METHOTREXATE | C20 H22 N8 O5 | 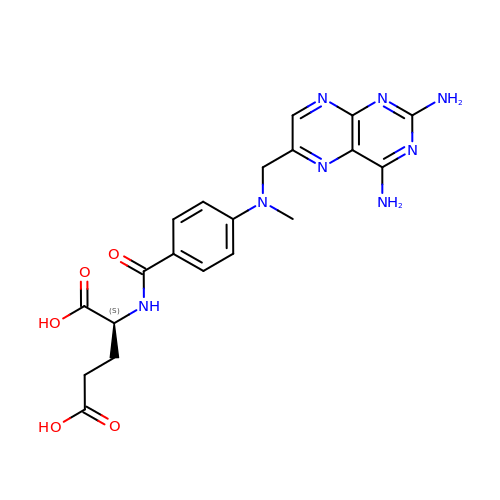FBOZXECLQNJBKD-ZDUSSCGKSA-N> MQIPASEQETLVRPKPELLKLLKSVGAQKDTYTMKE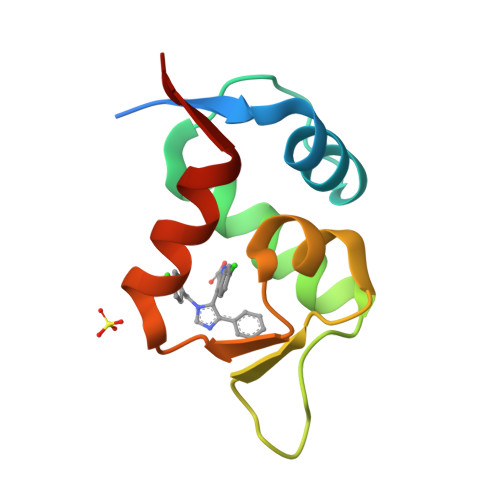VLFYLGQYIMTKRLYDEKQQHIVYCSNDLLGDLFGVPSFSVKEHRKIYTMIYRNLVVVN> MESDAKNYQIMDSWEEEPRDKSTNISSA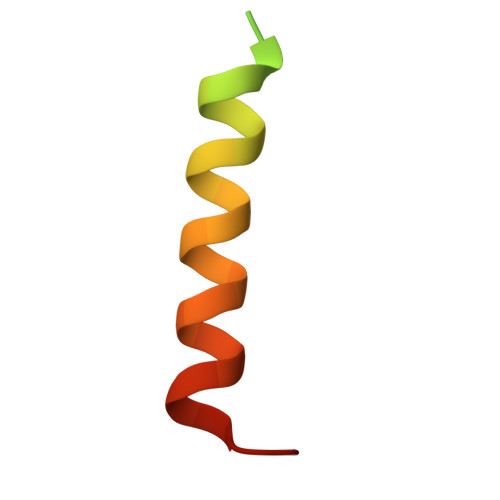LNIIEFILSTDPQE> MLRRCASAVAPAAHIPSPAAAVSGVQKRFLKIA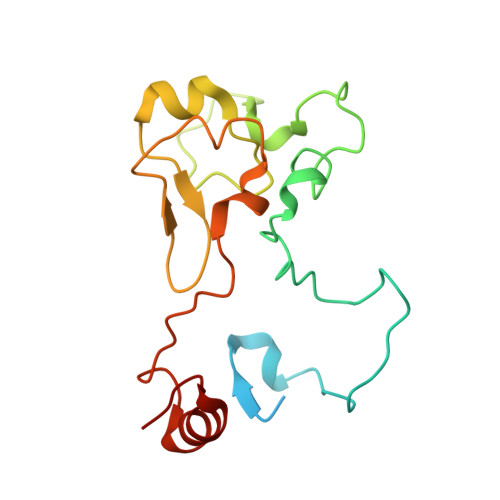KSTFGFYLARRGQRKFPFHRRPHIKNTQAMNLNAPYFWSYMTAKSQSFFLPEENYITGDWTGKFFVSKRQVYTLQHATSGGKVRVKSFPSVFELNSPSRWNVGKEMNTLTKPRMDLIDDQMLTKKQRLDYVKAGLLPK>[4x]MSNNIRIEEDLLGTREVPADAYYGVHTLRAIENFYISNNKISDIPEFVRGMVMVKKAAAMANKELQTIPKSVANAIIAACDEVLNNGKCMDQFPVDVYQGGAGTSVNMNTNEVLANIGLELMGHQKGEYQYLNPNDHVNKCQSTNDAYPTGFRIAVYSSLIKLVDAINQLREGFERKAVEFQDILKMGRTQLQDAVPMTLGQEFRAFSILLKEEVKNIQRTAELLLEVNLGAT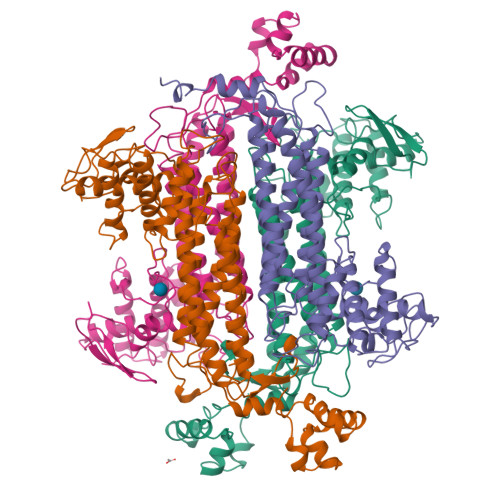AIGTGLNTPKEYSPLAVKKLAEVTGFPCVPAEDLIEATSDCGAYVMVHGALKRLAVKMSKICNDLRLLSSGPRAGLNEINLPELQAGSSIMPAKVNPVVPEVVNQVCFKVIGNDTTVTMAAEAGQLQLNVMEPVIGQAMFESVHILTNACYNLLEKCINGITANKEVCEGYVYNSIGIVTYLNPFIGHHNGDIVGKICAETGKSVREVVLERGLLTEAELDDIFSVQNLMHPAYKAKRYTDESEQ>[4x]NEIVVYSARADELLKPIAEAYQQKTGTKVTVVSDKAGPLMERLKAEGKNTQADVLITVDGGNLWQATQAGVLRPINSSVLKSNIPSHLRDPKNHWFGLSVRARTIFYNPNKVNPSELSTYADLADPKWKGRLCLRTSNNVYNQSLVATMIANHGQATTDRVVKGWVANLAAAPFANDTALLEAIDAGRCDVGIANTYYYGRLLNSKPQVANNVKVFFANQAGKGTHVNVSGAGVVKHSDNPAEAQKFIEWLSSNEAQRLYADRNFEYPANIQVTPTPAVARWGRFKQDFINVSVAGQNQQKAIMTMKRAGYK

Like MhFbpA and Thermus thermophilus FbpA (TtFbpA), McFbpA adopts a typical fold of class III periplasmic iron binding protein with the two globular lobes. Similar to other FbpA structures, McFbpA has two globular α/β domains named the N terminal lobe (Asn1-Trp95 and Val235-Val273) and the C terminal lobe (Tyr107-Ala221 and Thr274-Lys312). Each of the lobes consists of α helices surrounding a twisted mixed β sheet in the center. These two lobes are connected by a pair of antiparallel β strands (Phe96-Phe106 and Gly222-Val234), which acts as a hinge allowing for the adoption of either the open or closed conformation. Isogenic mutants of FbpA and AfeA were constructed, demonstrating that FbpA is essential for the utilization of human Tf and Lf as iron sources and that AfeA does not take up iron from these iron sources.

Our structural studies yielded the structure of M. catarrhalis FbpA in two different forms: an apo open form and an iron-holo open form. Comparisons with other FbpAs indicate that both iron-holo and apo McFbpA in this study are in the open conformation. The tyrosine residues (Tyr141, Tyr197 and Tyr198) are positioned in the same orientation as in other known structures, which classifies McFbpA as a class III iron-binding protein. The Fe–OH distances of Tyr141, Tyr197 and Tyr198 are 2.1 Å, 1.9 Å, and 2.1 Å, respectively. Analysis of electron density typical for metal ions, as illustrated in Fig. 4c, localizes the iron atom in the appropriate position. In the structure of iron-holo open McFbpA, we have determined that there are three tyrosine residues binding to the ferric ion and have confirmed that these residues are essential for the bacteria’s ability to utilize Tf and Lf as an iron source. There is additional electron density around the ferric ion in the structure, but it is indistinct for fitting waters and ligands. We believe that it might be multiple components from the crystallization condition that are non-specifically binding to the ferric ion, resulting in the electron density that is indistinct for any one component. In one of the four FbpA molecules in the holo crystal structure, we determined that two additional ferric ions are occupying the density surrounding the ferric ion bound by the three tyrosines. This might be caused by insufficient washing of the iron-bound protein, allowing for a slight excess amount of unbound ferric ion to remain with the protein.>[4x]PNQICLQKTTSTILKPRLISYTLPINTREGVCITDPLLAVDNGFFAYSHLEKIGSCTRGIAKQRIIGVGEVLD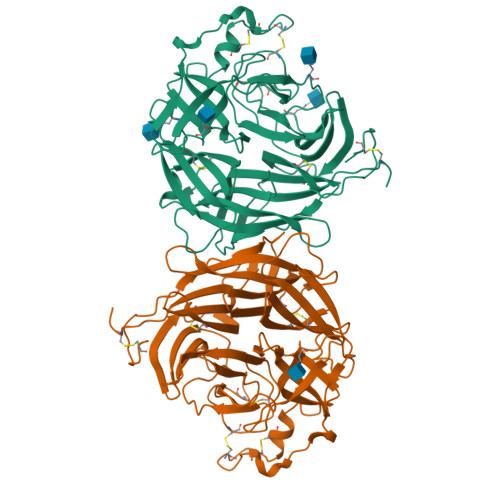RGDKVPSMFMTNVWTPPNPSTIHHCSSTYHEDFYYTLCAVSHVGDPILNSTSWTESLSLIRLAVRPKSDSGDYNQKYIAITKVERGKYDKVMPYGPSGIKQGDTLYFPAVGFLPRTEFQYNDSNCPIIHCKYSKAENCRLSMGVNSKSHYILRSGLLKYNLSLGGDIILQFIEIADNRLTIGSPSKIYNSLGQPVFYQASYSWDTMIKLGDVDTVDPLRVQWRNNSVISRPGQSQCPRFNVCPEVCWEGTYNDAFLIDRLNWVSAGVYLNSNQTAENPVFAVFKDNEILYQVPLAEDDTNAQKTITDCFLLENVIWCISLVEIYDTGDSVIRPKLFAVKIPAQCSES>[4x]MAWYEGAFFYQIFPDRFFRAGPPGRPAPAGPFEPWEAPPTLRGFKGGTLWGVAEKLPYLLDLGVEAIYLNPVFASTANHRYHTVDYFQVDPILGGNEALRHLLEVAHAHGVRV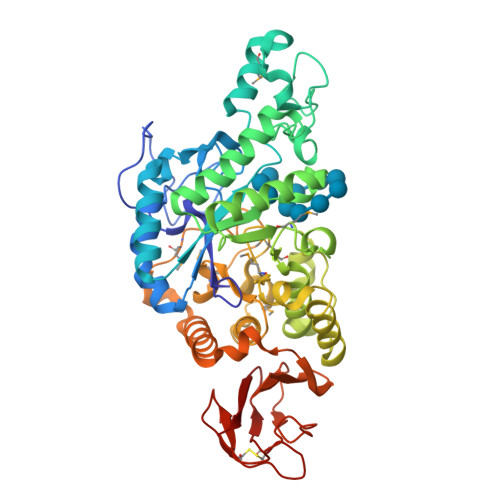ILDGVFNHTGRGFFAFQHLMENGEQSPYRDWYHVKGFPLKAYTAHPNYEAWWGNPELPKLKVETPAVREYLLAVAEHWIRFGVDGWRLDVPNEIPDPTFWREFRQRVKGANPEAYIVGEIWEEADFWLQGDMFDAVMNYPLARAVLGFVGGEALDRDLAAQTGLGRIEPLQALAFSHRLEDLFGRYRPEVVRAQMNLLTSHDTPRLLSLMRGSVERARLALALLFLLPGNPTVYYGEEVGMAGGKDPENRGGMVWEEARWQKDLRETVKRLARLRKEHPALRTAPYLRIYAQDGHLAFARGPYLAVVNASPHPFRQDFPLHGVFPRGGRAVDLLSGEVCTPQGGRLCGPVLPPFSLALWREA>[2x]MQAEKLGSEIKKIRVLRG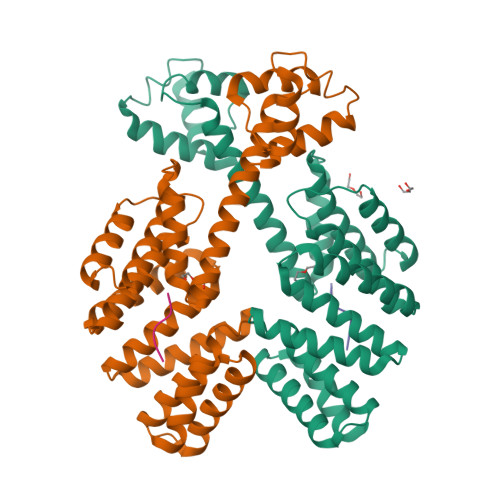LTQKQLSENICHQSEVSRIESGAVYPSMDILQGIAAKLQIPIIHFYEVLIYSDIERKKQFKDQVIMLCKQKRYKEIYNKVWNELKKEEYHPEFQQFLQWQYYVAAYVLKKVDYEYCILELKKLLNQQLTGIDVYQNLYIENAIANIYAENGYLKKGIDLFEQILKQLEALHDNEEFDVKVRYNHAKALYLDSRYEESLYQVNKAIEISCRINSMALIGQLYYQRGECLRKLEYEEAEIEDAYKKASFFFDILEMHAYKEALVNKISRLEHHHHHH;>LPFEF[2x]>NRSLNELSLSDILIAADVEGGLHAVDRRNGHIIWSIEPENFQPLIEIQEPSRLETYETLIIEPFGDGNIYYFNAHQGLQKLPLSIRQLVSTSPLHLKTNIVVNDSGKIVEDEKVYTGSMRTIMYTINMLNGEIISAFGPGSKNGYFGSQSVDCSPEEKIKLQECENMIVIGKTIFELGIHSYDGASYNVTYSTWQQNVLDVPLALQNTFSKDGMCIAPFRDKSLLASDLDFRIARWVSPTFPGIIVGLFDVFNDLRTNENILVPHPFNPGDHESISSNK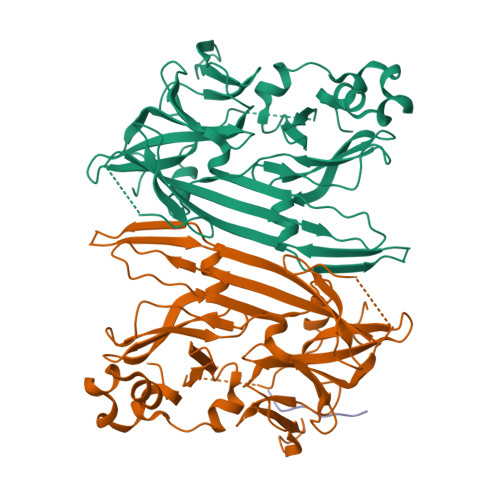VYLDQTSNLSWFALSSQNFPSLVESAPISRYASSDRWRVSSIFEDETLFKNAIMGVHQIY[2x];> VVVVVVVV> LDDFQKEEQAVNQEEKEQKLQFVLRFGDFEDVISLSKLNVNGSKTTLYSFENRYYL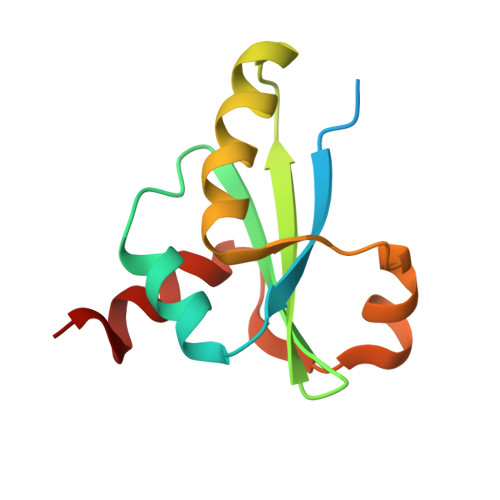YVDFCNMTDEEVENQLSILLEYATESSISIHRLEEYGKLIISEHALETIKKHFAS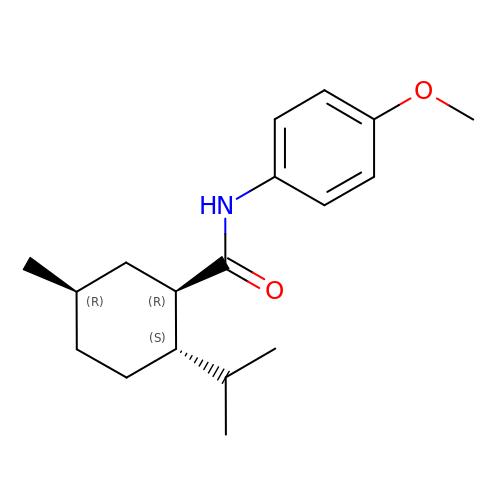(1R,2S,5R)-N-(4-methoxyphenyl)-5-methyl-2-(propan-2-yl)cyclohexane-1-carboxamide | C18 H27 N O2 | HNSGVPAAXJJOPQ-XOKHGSTOSA-N>GSKRLISLCVGCGNQIHDQYILRVSPDLEWHAACLKCAECNQYLDESCTCFVRDGKTYCKRDYIRLYGIKCAKCSIGFSKNDFVMRARSKVYHIECFRCVACSRQLIPGDEFALREDGLFCRADHDVVERGGSGGHMGSGGGDVMVVGEPTLMGGEFGDEDERLITRLENTQF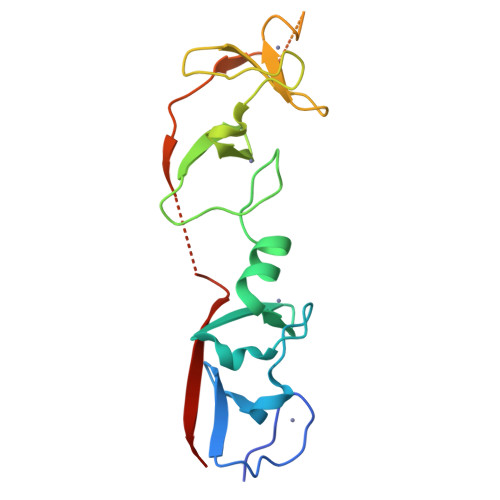[3x]>MSGNEREKVKTVPLHLEEDIRPEMKEDIHDPTYQDEEGPPPKLEYVWRNIILMVLLHLGGLYGIILVPSCKLYTCLFGIFYYMTSALGITAGAHRLWSHRTYKARLPLRIFLIIANTMAFQNDVYEWARDHRAHHKFSETHADPHNSRRGFFFSHVGWLLVRKHPAVKEKGGKLDMSDLKAEKLVMFQRRYYKPGLLLMCFILPTLVPWYCWGETFVNSLFVSTFLRYTLVLNATWLVNSAAHLYGYRPYDKNIQSRENILVSLGAVGEGFHNYHHTFPFDYSASEYRWHINFTTFFIDCMAALGLAY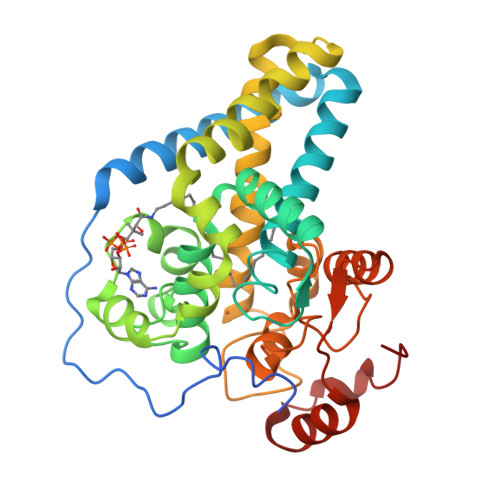DRKKVSKATVLARIKRTGDGSHKSSENLYFQ[2x]(1~{S},2~{S})-2-[5-[cyclopropylmethyl(naphthalen-1-yl)amino]-4-methoxy-pyrimidin-2-yl]carbonylcyclopropane-1-carboxylic 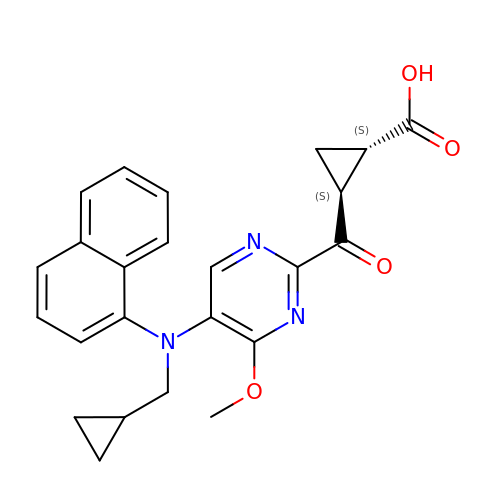acid | C24 H23 N3 O4 | QYPOYXFLLPVCEL-ROUUACIJSA-N> SQAATPAADGKVKISIDPLTRVEGHLKIEVEVKDGKVVDAKCSGGMFRGFEQILRGRDPRDSSQIVQRICGVCPTAHCTASVMAQDDAFGVKVTTNGRITRNLIFGANYLQSHILHFYHLAALDYVKGPDVSPFVPRYANADLLTDRIKDGAKADATNTYGLNQYLKALEIRRICHEMVAMFGGRMPHVQGMVVGGAT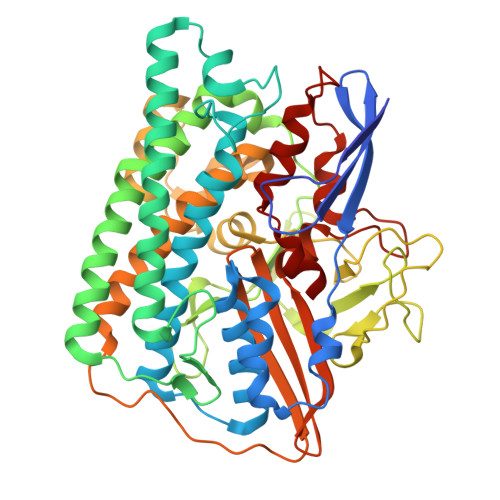EIPTADKVAEYAARFKEVQKFVIEEYLPLIYTLGSVYTDLFETGIGWKNVIAFGVFPEDDDYKTFLLKPGVYIDGKDEEFDSKLVKEYVGHSFFDHSAPGGLHYSVGETNPNPDKPGAYSFVKAPRYKDKPCEVGPLARMWVQNPELSPVGQKLLKELYGIEAKKFRDLGDKAFSIMGRHVLRAEETWLTAVAVEKWLKQVQPGAETYVKSEIPDAAEGTGFTEAPRGALLHYLKIKDKKIENYQIVSATLWNANPRDDMGQRGPIEEALIGVPVPDIKNPVNVGRLVRSYDPULGCAVH>[2x]MKTKFCTGGEAEPSPLGLLLSCGSGSAAPAPGVGQQRDAASDLESKQLGGQQPPLALPPPPPLPLPLPLPQPPPPQPPADEQPEPRTRRRAYLWCKEFLPGAWRGLREDEFHISVIRGGLSNMLFQCSLPDTTATLGDEPRKVLLRLYGAILQMRSCNKEGSEQAQKENEFQGAEAMVLESVMFAILAERSLGPKLYGIFPQGRLEQFIPSRRLDTEELSLPDISAE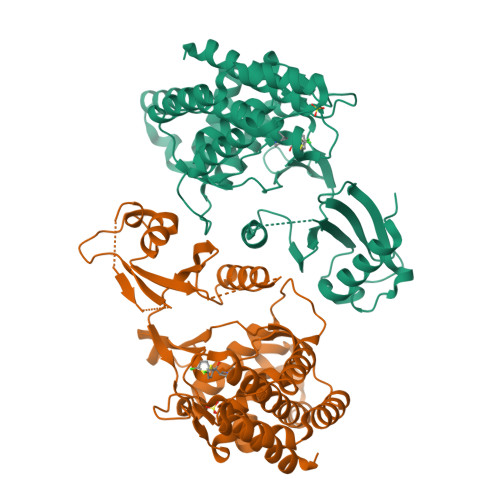IAEKMATFHGMKMPFNKEPKWLFGTMEKYLKEVLRIKFTEESRIKKLHKLLSYNLPLELENLRSLLESTPSPVVFCHNDCQEGNILLLEGRENSEKQKLMLIDFEYSSYNYRGFDIGNHFCEWMYDYSYEKYPFFRANIRKYPTKKQQLHFISSYLPAFQNDFENLSTEEKSIIKEEMLLEVNRFALASHFLWGLWSIVQAKISSIEFGYMDYAQARFDAYFHQKRKLGV> SNAASGSALIFDEEMSRYKLLWTDPECEIEVPERLTVSYEALRTHGLAQRCKAVPVRQATEQEILLAHSEEYLEAVKQTPGMNVEELMAFSKKYNAVYFHQNIYHCAKLAAGATLQLVDSVMKREVRNGMALVRPPGHHSQRSAANGFCVFNNVAFAALYAKKNYNLNRILIVDWDVHHGQGIQYCFEEDPSVLYFSWHRYEHQSFWPNLPESDYSSVGKGKGSGFNINLPWNKVGMTNSDYLAAFFHVLLPVAYEFDPELVIVSAGFDSAIGDPEGEMCALPEIFAHLTHLLMPLAAGKMCVVLEGGFNLTSLGQSVCQTVHSLLGDPTPRISGLGTACDSALESIQNVRNVQSSYWSSFKHLAQSETNPKRPRLDATNGGPKESSEPASESNPKKTAQDIVWPEPLKRMPASVRTVVVPPPGVELTLPKNCQHSGDISESTAKEVQRIRDKHFHDLTDQNILRSLGNIISVLDRMMRSDEVCNGCVVVSDLSVSVQCALQHALTEPAERVLVVYVGDGELPVKTNDGKVFLVQICTKETEDKCVNRLTLCLREGESLTAGFMQALLGLILPVAYEFNPALVLGIVE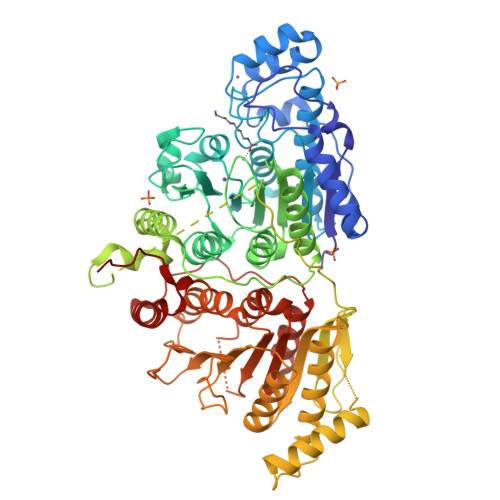ETAAKTRLMRVWGHMTCLIQGLARGRMLTLLQGYDKDLLELTVSALSGASISPLGPLRAPKPEDVEMMEKQRQRLQERWGLLRCTVSESW>RKPKTGILMLNMGGPETLGDVHDFLLRLFLDRDLMTLPIQNKLAPFIAKRRTPKIQEQYRRIGGGSPIKIWTSKQGEGM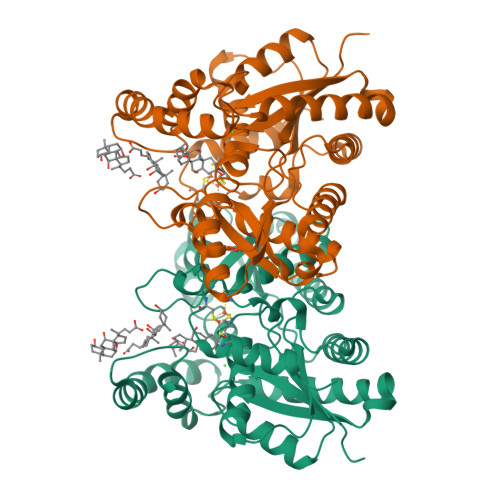VKLLDELSPNTAPHKYYIGFRYVHPLTEEAIEEMERDGLERAIAFTQYPQYSCSTTGSSLNAIYRYYNQVGRKPTMKWSTIDRWPTHHLLIQCFADHILKELDHFPLEKRSEVVILFSAHSLPMSVVNRGDPYPQEVSATVQKVMERLEYCNPYRLVWQSKVGPMPWLGPQTDESIKGLCERGRKNILLVPIARTSDHIETLYELDIEYSQVLAKECGVENIRRAESLNGNPLFSKALADLVHSHIQSNELCSKQLTLSCPLCVNPVCRETKSFFTSQQL[2x]> NTYQFRNMIECTVPSRSWWDFADYGCYCGCGSGT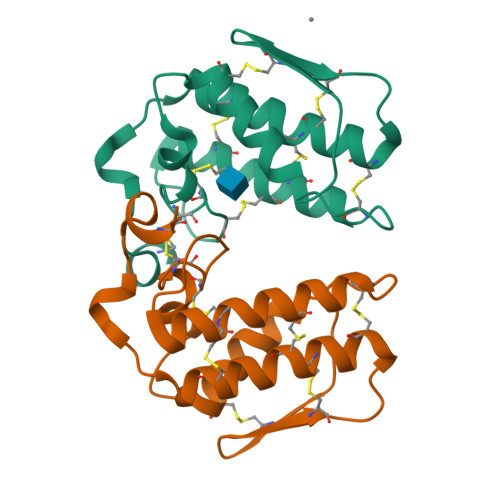PTDDLDRCCQVHCNCYRQAGEISGCRPKFKTYTYQCSGGTLTCKGNNNACAASSCDCDRLAAICFAGAPYNDNNYNIDLKARCN;> NIKQFNNMIECTVPARSWWDFADYGCYCGSGSGSPTDDLDRCCQTHDNCYGAGGGSTGCAPKSRTYTYQCSQGTLTCSGENSACAATTCDCDRLAAICFAGAPYNDTNYNIDLKSRCQ> 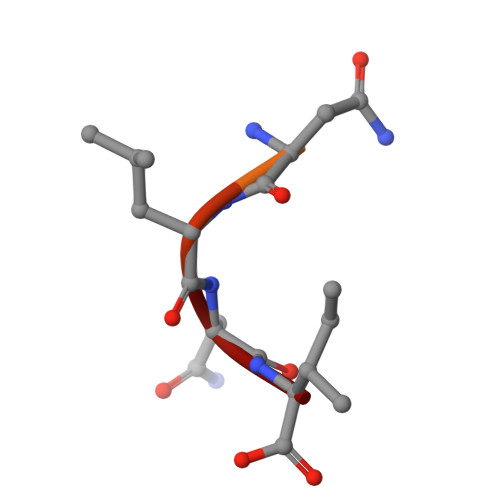GIDDGMNLNI>MSLVVFPFKHEHPEVLLHNVRVAAAHPRVHEVLCIGYERDQTYEAVERAAPEISRATGTPVSVRLQERLGTLRPGKGDGMNTALRYFLEETQWERIHFYDADITSFGPDWITKAEEAADFGYGLVRHYFPRASTDAMITWMITRTGFALLWPHTELSWIEQPLGGELLMRREVAAMLYEDERVRRRSDWGIDTLYTFVTVQQGVSIYECYIPEGKAHRLYGGLDDLRTMLVECFAAIQSLQHEVVGQPAIHRQEHPHRVPVHIAERVGYDVEATLHRLMQHWTPRQVELLELFTTPVREGLRTCQRRPAFNFMDEMAWAATYHVLLEHFQPGDPDWEELLFKLWTTRVLNYTMTVAL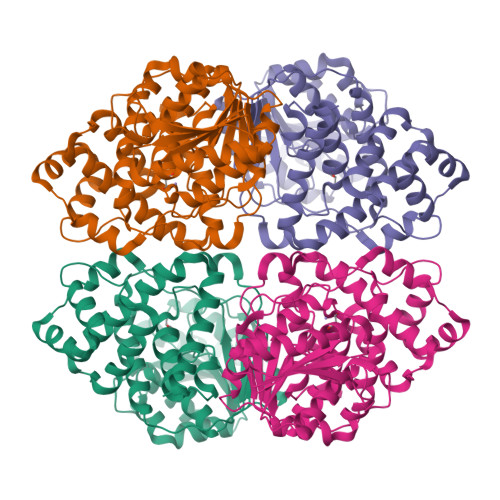RGYDYAQQYLYRMLGRYRYQAALENGRGHPVPPRAALSTA[2x]> NSINDSKILSLQNKKNTLMDTSGYNAEVRVEGNVQLNPIFPFDFKLGSSGDDRGKVIVTQNENIVYNAMYESFSISFWIRINKWVSNLPGYTIIDSVKNNSGWSIGIISNFLVFTLKQNENSEQDINFSYDISK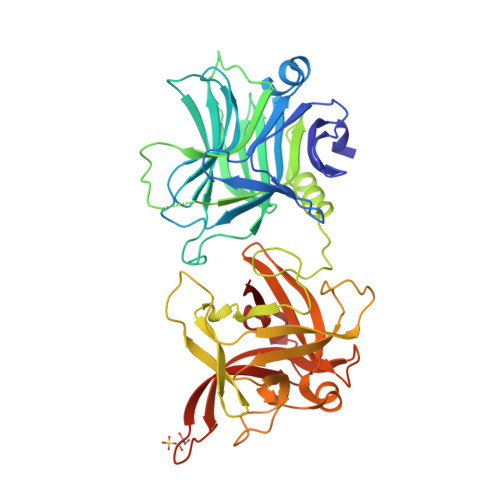NAAGYNKWFFVTITTNMMGNMMIYINGKLIDTIKVKELTGINFSKTITFQMNKIPNTGLITSDSDNINMWIRDFYIFAKELDDKDINILFNSLQYTNVVKDYWGNDLRYDKEYYMINVNYMNRYMSKKGNGIVFNTRKNNNDFNEGYKIIIKRIRGNTNDTRVRGENVLYFNTTIDNKQYSLGMYKPSRNLGTDLVPLGALDQPMDEIRKYGSFIIQPCNTFDYYASQLFLSSNATTNRLGILSIGSYSFKLGDDYAFNHEYLIPVIKIEHYASLLESTSTHWVFVPASE> MGSDKIHHHHHHMDELLEKAKKVREAWDVLRNATTREKNKAI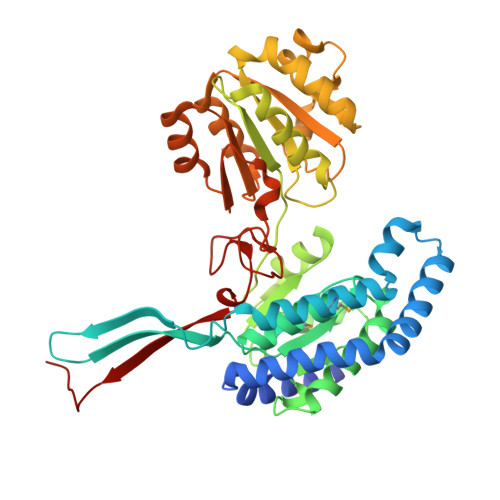KKIAEKLDERRKEILEANRIDVEKARERGVKESLVDRLALNDKRIDEMIKACETVIGLKDPVGEVIDSWVREDGLRIARVRVPIGPIGIIYESRPNVTVETTILALKSGNTILLRGGSDALNSNKAIVSAIREALKETEIPESSVEFIENTDRSLVLEMIRLREYLSLVIPRGGYGLISFVRDNATVPVLETGVGNCHIFVDESADLKKAVPVIINAKTQRPGTCNAAEKLLVHEKIAKEFLPVIVEELRKHGVEVRGCEKTREIVPDVVPATEDDWPTEYLDLIIAIKVVKNVDEAIEHIKKYSTGHSESILTENYSNAKKFVSEIDAAAVYVNASTRFTDGGQFGFGAEIGISTQRFHARGPVGLRELTTYKFVVLGEYHVRE>GATADRDILARLHKAVTSHYHAITQEFENFDTMKTNTISREEFRAICNRRVQILTDEQFGRLWNEMPVNAKGRLKYPDFLSRFSSETAATP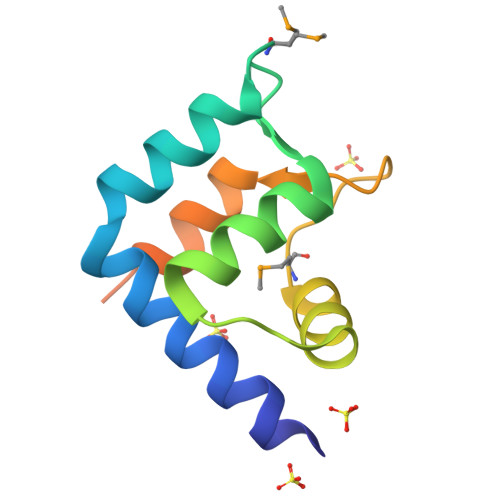MATGDSAVAQR[4x]>ACCC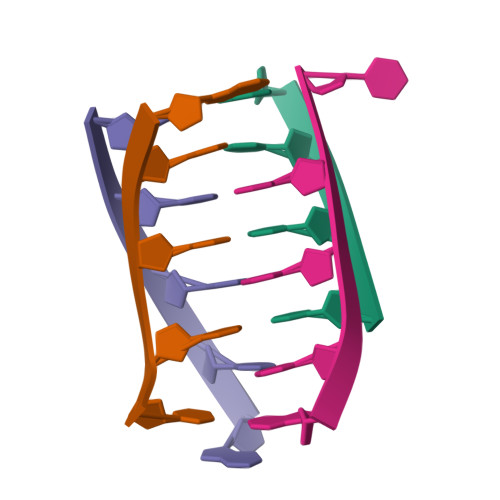T[4x]>PQSQKI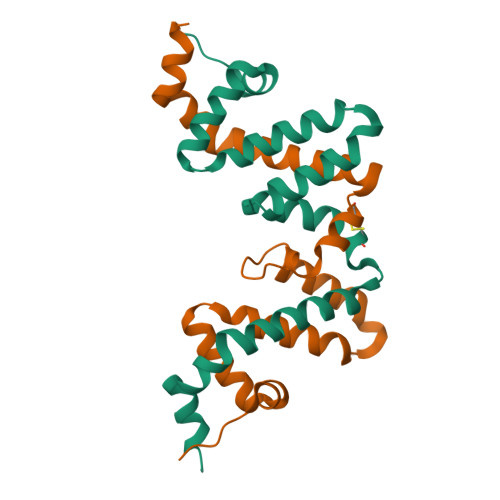LQFEDIMTNPFYRERFGTYMERIDKRALVGFWESAEHLKNANKSEIPQLVSEMYQNFFVESKEISVEKSLYKEIQQCLVGNRGIEVFSKIQADVSEVLRERYYPSFLVSDLYEKLMREEE[2x]> METAIITLSKDGRITEWNKKAEQLFGLKKENVLGRRLKDLPDFEEIG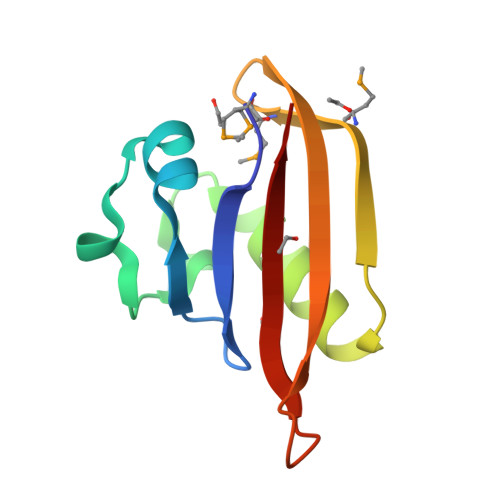SVAESVFENKEPVFLNMYKMGERYFNIRFSPFRNAKTQLLEGVIITIDD> SERAYNFNAGPAALPLEVLERAQAEFVDYQHTGMSIMEMSHRGAVYEAVHNEAQARLLALLGNPTGYKVLFIQGGASTQFAMIPMNFLKEGQTANYVMTGSWASKALKEAKLIGDTHVAASSEASNYMTLPKLQEIQL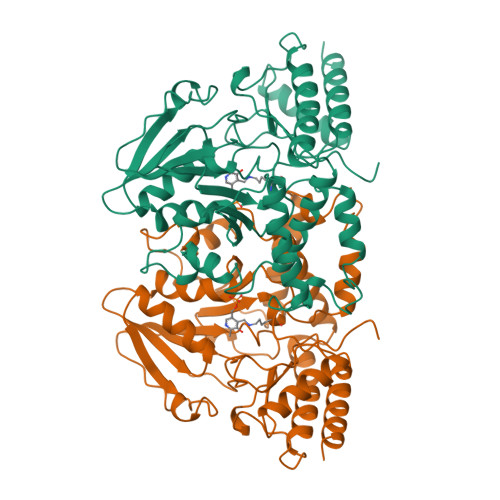QDNAAYLHLTSNETIEGAQFKAFPDTGSVPLIGDMSSDILSRPFDLNQFGLVYAGAQKNLGPSGVTVVIVREDLVAESPKHLPTMLRYDTYVKNNSLYNTPPSFGIYMVNEVLKWIEERGGLEGVQQANRKKASLIYDAIDQSGGFYRGCVDVDSRSDMNITFRLASEELEKEFVKASEQEGFVGLKGHRSVGGLRASIYNAVPYESCEALVQFMEHFKRSRG In a search for putative DNA-binding domains, BurrH, a protein that recognizes a 19 bp DNA target, was identified. Here, its apo and DNA-bound crystal structures are reported, revealing a central region containing 19 repeats of a helix–loop–helix modular domain (BurrH domain; BuD), which identifies the DNA target by a single residue-to-nucleotide code, thus facilitating its redesign for gene targeting. We identified BurrH in Burkholderia rhizoxinica, a symbiotic bacterium found in the cytosol of Rhizopus microspores. Each BuD repeat is composed of 33 residues, only eight of which are strictly conserved between the repeats.

We expressed, purified and solved the structure of this protein, which is able to specifically recognize its DNA target. The models were refined to 2.21 and 2.65 Å resolution, respectively. BurrH shrinks 23 Å along the longitudinal axis wrapping the DNA molecule, which displays an almost unperturbed B-form.

>STAFVDQDKQMANRLNLSPLERSKIEKQYGGATTLAFISNKQNELAQILSRADILKIASYDCAAHALQAVLDCGPMLGKRGFSQSDIVKIAGNIGGAQALQAVLDLESMLGKRGFSRDDIAKMAGNIGGAQTLQAVLDLESAFRERGFSQADIVKIAGNNGGAQALYSVLDVEPTLGKRGFSRADIVKIAGNTGGAQALHTVLDLEPALGKRGFSRIDIVKIAANNGGAQALHAVLDLGPTLRECGFSQATIAKIAGNIGGAQALQMVLDLGPALGKRGFSQATIAKIAGNIGGAQALQTVLDLEPALCERGFSQATIAKMAGNNGGAQALQTVLDLEPALRKRDFRQADIIKIAGNDGGAQALQAVIEHGPTLRQHGFNLADIVKMAGNIGGAQALQAVLDLKPVLDEHGFSQPDIVKMAGNIGGAQALQAVLSLGPALRERGFSQPDIVKIAGNTGGAQALQAVLDLELTLVEHGFSQPDIVRITGNRGGAQALQAVLALELTLRERGFSQPDIVKIAGNSGGAQALQAVLDLELTFRERGFSQADIVKIAGNDGGTQALHAVLDLERMLGERGFSRADIVNVAGNNGGAQALKAVLEHEATLNERGFSRADIVKIAGNGGGAQALKAVLEHEATLDERGFSRADIVRIAGNGGGAQALKAVLEHGPTLNERGFNLTDIVEMAANSGGAQALKAVLEHGPTLRQRGLSLIDIVEIASNGGAQALKAVLKYGPVLMQAGRSNEEIVHVAARRGGAGRIRKMVAPLLERQGGSEFELENLYFQGELRRQASALE[2x]> SMHSDLTFCEIILMEMESHDAAWPFLEPVNPRLVSGYRRIIKNPMDFSTMRHRLSRGGYTSSEEFAADALLVFDNCQTFNEDDSEVGKAGHIMRRFFESRWEEFY

BAZ2A is an epigenetic regulator affecting transcription of ribosomal RNA. It is overexpressed in aggressive and recurrent prostate cancer, promoting cellular migration. BAZ2A, however, features a shallow pocket, making it one of the least druggable bromodomains. Here, we describe a structure-based fragment-growing campaign for the identification of ligands of the BAZ2A bromodomain.

The 3-aminopropyl substituent in compound 44 performs better than the N-methyl-2-aminoethyl group of 45. Binding poses of compounds 44 and 45 are similar: all interactions of the acetyl-pyrrole headgroup are conserved with respect to 25, but the charged tails do not point toward Trp1816, but instead approach Glu1820. However, as observed in compound 36, Glu1820 oscillates between two conformers, one in contact with the compound amino group and the other exposed to the solvent; this interaction seems to contribute only partially to the binding affinity. Instead, compound 44 is involved in a network of water-mediated interactions with the protein matrix. The thiazole nitrogen forms a hydrogen bond with water W4, which tetrahedrally interacts with the main chain of Pro1817 and water molecules W5 and W6, in turn in contact with BAZ2A. Water W5 is tetrahedrally coordinated by the terminal amino group of 44, the Trp1816 main-chain oxygen, the Leu1819 main-chain nitrogen, and W4. Despite the observed interaction patterns, both compounds have poor affinity for BAZ2A, most probably due to the entropic penalty deriving from the freezing of the alkylamine tails and the surrounding water network. Notably, in the structures in complex with 44, 45, and 47, an ethylene glycol molecule is sandwiched between the thiazole ring and the ZA loop. It forms a hydrogen bond with the main-chain nitrogen of Asn1823, an important anchoring point already explored by the BAZ-ICR and GSK2801 chemical probes and other BAZ2A inhibitors, and a relevant indication for further optimization of this chemical class.> GSRTGSESSRPNTALLDPSSPEFSAVVSVGDWLQAIKMDRYKDNFTAAGYTTL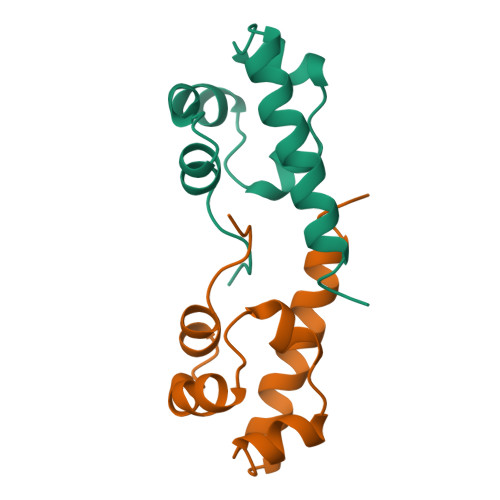EAVVHMSQDDLARIGITAITHQNKILSSVQAMRTQMQQMHG>SEITKTLLNIRSLRAYARELTIEQLEEALDK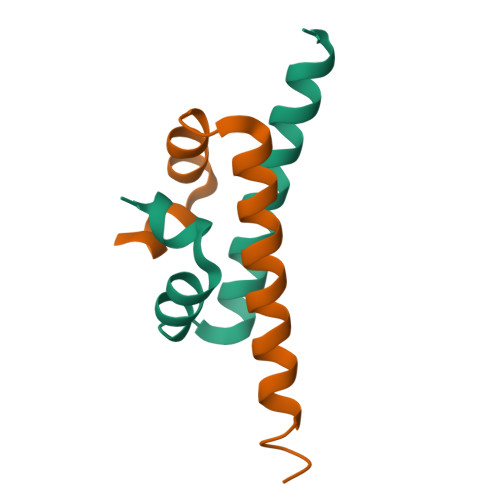LTTVVQERKEAEAEEIAAR[2x]(1R,2R,3S,4R,6S)-4,6-diamino-2,3-dihydroxycyclohexyl 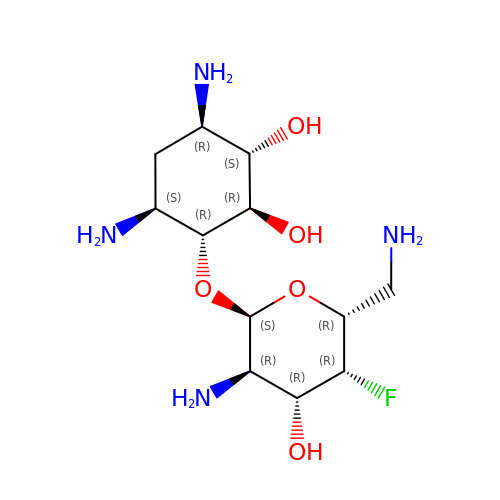2,6-diamino-2,4,6-trideoxy-4-fluoro-alpha-D-galactopyranoside | C12 H25 F N4 O5 | CRXNRBKQEXVRGM-RMDUJVAESA-N> MTSRVDPANPGSELDSAIRDTLTYSNCPVPNALLTASESGFLDAAGIELDVLSGQQGTVHFTYDQPAYTRFGGEIPPLLSEGLRAPGRTRLLGITP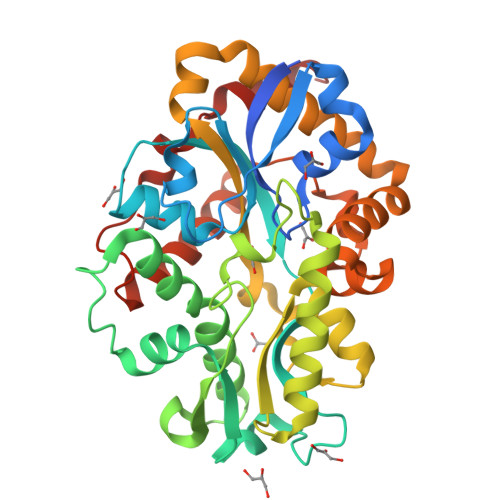LLGRQGFFVRDDSPITAAADLAGRRIGVSASAIRILRGQLGDYLELDPWRQTLVALGSWEARALLHTLEHGELGVDDVELVPISSPGVDVPAEQLEESATVKGADLFPDVARGQAAVLASGDVDALYSWLPWAGELQATGARPVVDLGLDERNAYASVWTVSSGLVRQRPGLVQRLVDAAVDAGLWARDHSDAVTSLHAANLGVSTGAVGQGFGADFQQRLVPRLDHDALALLERTQQFLLTNNLLQEPVALDQWAAPEFLNNSLNRHR> GHPYYLRSFLVVLKTVLENEDDMLLFDEQEKGIVTKFYQLSATGQKLYVRLFQRKLSWIKMTKLEYEEIALDLTPVIEELTNAGFLQTESELQELSEVLELLSAPELKSLAKTFHLVNPNGQKQQLVDAFLKLAKQRSVCTWGKNKPGIGAVILKRAKALAGQSVRICKGPRAVFSRILLLFSLTDSMEDEDAACGGQGQLSTVLLVNLGRMEFPSYTINRKTHIFQDRDDLIRYAAATHMLSDISSAMANGNWEEAKELAQCAKRDWNRLKNHPSLRCHEDLPLFLRCFTVGWIYTRILSRFVEILQRLHMYEEAVRELESLLSQRIYCPDSRGRWWDRLALNLHQHLKRLEPTIKCITEGLADPEVRTGHRLSLYQRAVRLRESPSCKKFKHLFQQLPEMAVQDVKHVTITGRLCPQRGMCKSVFVMEAGEAADPTTVLCSVEELALAHYRRSGFDQGIHGEGSTF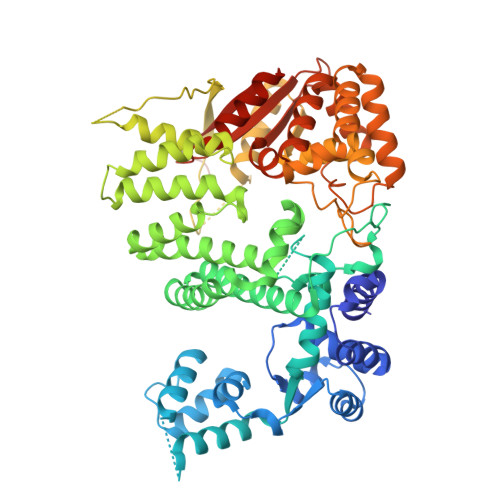STLYGLLLWDIIFMDGIPDVFRNACQAFPLDLCTDSFFTSRRPALEARLQLIHDAPEESLRAWVAATWHEQEGRVASLVSWDRFTSLQQAQDLVSCLGGPVLSGVCRHLAADFRHCRGGLPDLVVWNSQSRHFKLVEVKGPNDRLSHKQMIWLAELQKLGAEVEVCHVVAVGGSENLYFQ> GSFVGSIDQGTTSSRFLIFNGEGNPVASHQIE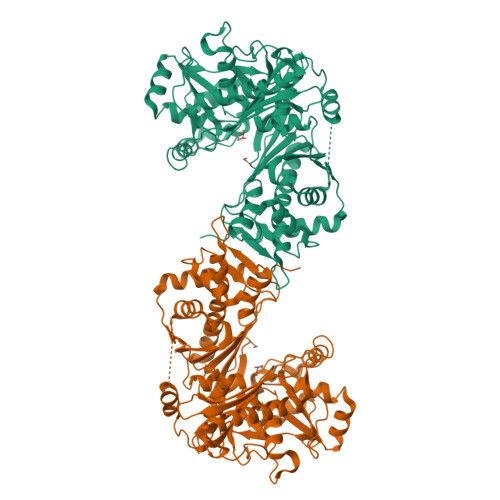FENLYPKSGWHEQDPYELLNSVQQCIDGAMHKFASLGYSKENIRAIGITNQRETTVVWDSVTGEPLHNAIVWPDTRTSALVRELKARQSADSLLELCGLPLSTYPSSVKLLWLIQNVDAVKQAYEEGRLAFGTVDSWLIYKLNGGAQAERPIHVTDSTNASRTMFMNLRTLQYDDKLLGFFGIDRNKIKLPKIVPSSDPEAFGKVATGALAGVPIAGCLGDQSSALVGQCGFSPGQAKNTYGTGCFLLYNVGTEPVISKYGLLATVAYDFGRGRKPVYALEGSIAVAGAGITFLMNNLGFAPKPSEINALAESVLDNGGVVFVTAFSGLFAPYWIDDAKGTLFGITQHTTKGHIARATLEATCYQTRAILDAMEKDSGHKLESLAVDGGLSASDLCMQTQADISGIPVDRPRMRETTALGAAIAAGLATGVWRELDHVKESIAGGANGNGKKNAREVFYPKMDRKKAERLFRKWEQAVEMSRGWVREQEEEDGE> MGHHHHHHSQDPNSNVTLTAVKKAFPDALTNAELVAMVSKRLSQFGYHKYNTLLATSLCRDEVTRPLEQDFGEVYGKHFTMGGLAGFPFGGLTGFGAMAGHIPDGGSCLLIYGSHVGVSWEGKWGTVARRGREKGGACCGS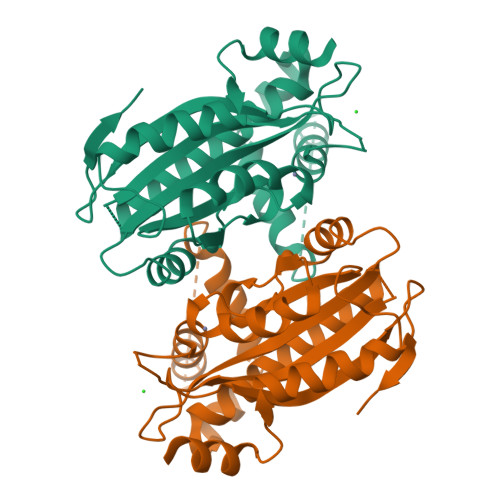AVAAAQAVTQAYQATLDESSSSSSSSATSTPVYRYSNDPLDAQQGYVRDMLRPYAATLSEAEDVMVTLPVSVYDAQQKLVTRILDEGSNHIDGDGQIAVVGGIQINTPKEMSDFFVVRRFCIRDSSGNMVENFMPLTAGRE>[2x]MDAQSAAKCLTAVRRHSPLVHSITNNVVTNFTANGLLALGASPVMAYAKEEVADMAKIAGALVLNIGTLSKESVEAMIIAGKSANEHGVPVILDPVGAGATPFRTESARDIIREVRLAAIRGNAAEIAHTVGVTDWLIKGVDAGEGGGDIIRLAQQAAQKLNTVIAITGEVDVIADTSHVYTLHNGHKLLTKVTGAGCLLTSVVGAFCAVEENPLFAAIAAISSYGVA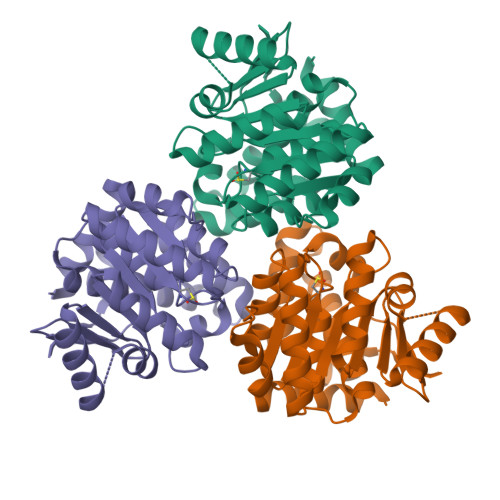AQLAAQQTADKGPGSFQIELLNKLSTVTEQDVQEWATIERVTVS> VLHQPPAMSSALGTTIRLTCTLRNDHDIGVYSVYW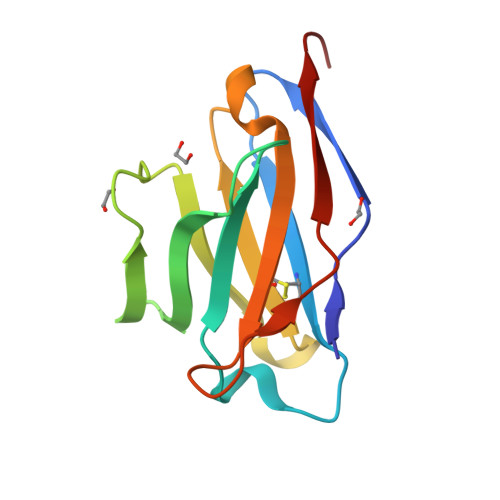YQQRPGHPPRFLLRYFSQSDKSQGPQVPPRFSGSKDVARNRGYLSISELQPEDEAMYYCAMGARSTHVFGSGTQLTVLSAA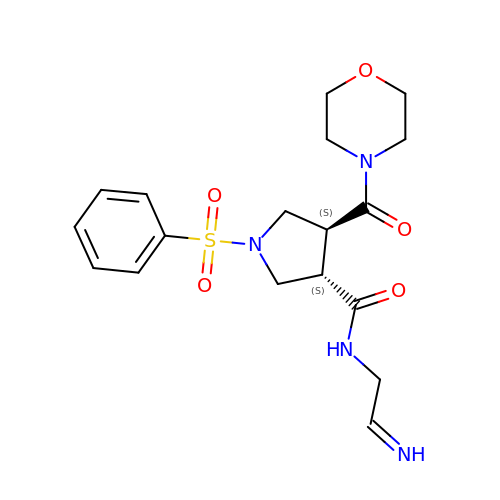(3S,4S)-N-[(2E)-2-iminoethyl]-4-(morpholin-4-ylcarbonyl)-1-(phenylsulfonyl)pyrrolidine-3-carboxamide | C18 H24 N4 O5 S | WRVODTAPCBNKHV-DRTXVBNMSA-N> MAVELPKAAIERIFRQGIGERRLSQDAKDTIYDFVPTMAEYVANAAKSVLDASGKKTLMEEHLKALADVLMVEGVEDYDGELFGRATVRRILKRAGIERASSDAVDLYNKLICRATEELGEKAAEYADEDGRKTVQGED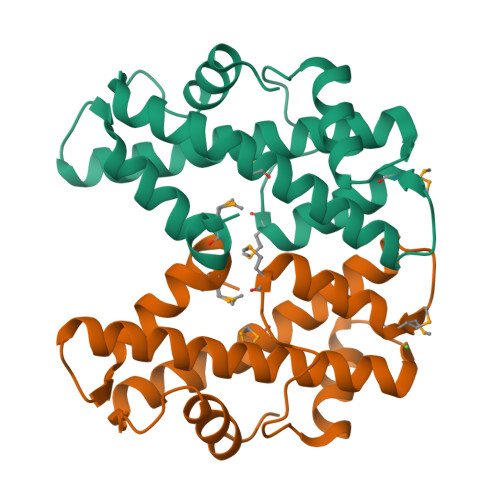VEKAITYSMPKGGEL> MSEKPAESAAAVADSATTTAPQSGKPETALPALIDTQATAETRALYRNLAKLRYKHLLFGHEDSLAYGVHWEGDMDRSDVRDVTGANPAVYGWELGGLELGHTANLDAVNFEKMQHWIKAGYSRGGVITISWHVFNPVSGGNSWDKTPAVHELIPGGARHATLKAYLDTFVAFNEGLADVDAQGNKHYPPIIFRPWHEHNGDWFWWGKGHASEQDYIALWRFTVHYLRDEKKLRNLIYAYSPDRSRIDMANFEAGYLYGYPGDAYVDIIGLDNYWDVGHEANTASADEQKAALTASLKQLVQIARSKGKIAALTETGNNRLTIDNFWTERLLGPISADADASEIAYVMVWRNANLAREKSEQFFAPFPGQATADDFKRFYQS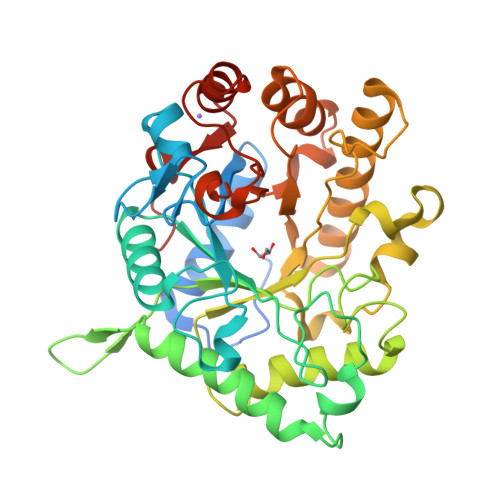EVVLFEDELPPLYR>SRKFFVGGNWKMNGRKQSLGELIGTLNAAKVPADTEVVCAPPTAYIDFARQKLDPKIAVAAQNCYKVTNGAFTGEISPGMIKDCGATWVVLGHSERRHVFGESDELIGQKVAHALAEGLGVIACIGEKLDEREAGITEKVVFEQTKVIADNVKDWSKVVLAYEPVWAIGTGKTATPQQAQEVHEKL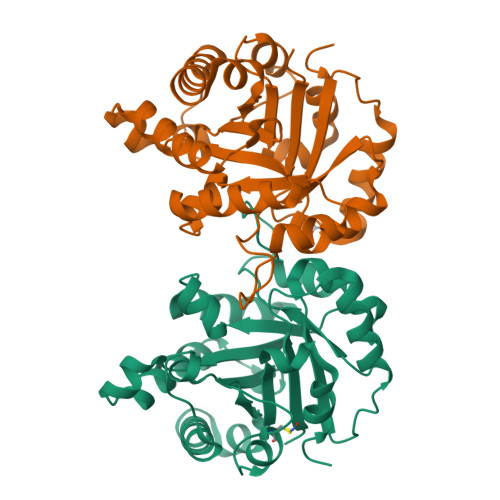RGWLKSNVSDAVAQSTRIIYGGSVTGATCKELASQPDVDGFLVGGASLKPEFVDIINAKQ[2x]>MSPTTDRIAVVGGSISGLTAALMLRDAGVDVDVYERSPQPLSGFGTGIVVQPELVHYLLEQGVELDSISVPSSSMEYVDALTGERVGSVPADWRFTSYDSIYGGLYELFGPERYHTSKCLVGLSQDSETVQMRFSDGTKAEANWVIGADGGASVVRKRLLGIEPTYAGYVTWRGVLQPGEVADDVWNYFNDKFTYGLLDDGHLIAYPIPGRENAESPRLNFQWYWNVAEGPDLDELMTDVRGIRLPTSVHNNSLNPHNLRQFHSKGESLFKPFRDLVLNASSPFVTVVADATVDRMVHGRVLLIGDAAVTPRPHAAA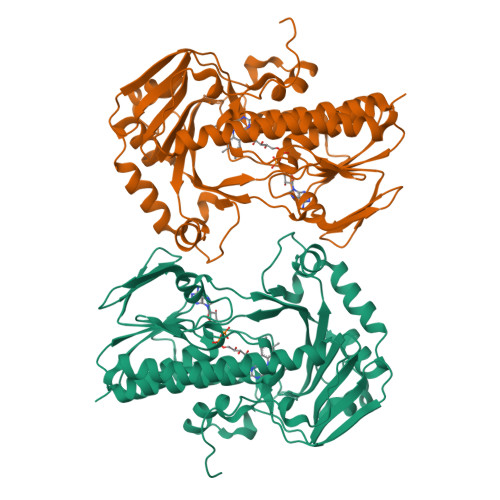GGAKASDDARTLAEVFTKNHDLRGSLQSWETRQLQQGHAYLNKVKKMASRLQHGGSFEPGNPAFAFGLPKVDEPSVVTNS[3x]> MSFTNVNYPASDGTVIFTEEQEALVVQSWNVMKKNSAELGLKLFLKIFEIAPTAKKMFSFVRDSDVPLEQNQKLKGHAMSVFVMTCKSAAQLRKAGKVTFGESSLKHMGSVHLKYGVVDEHFEVTRFALLETIKEAVPEMWSPEMKNAWAEAFNHLVAAIKAEMQR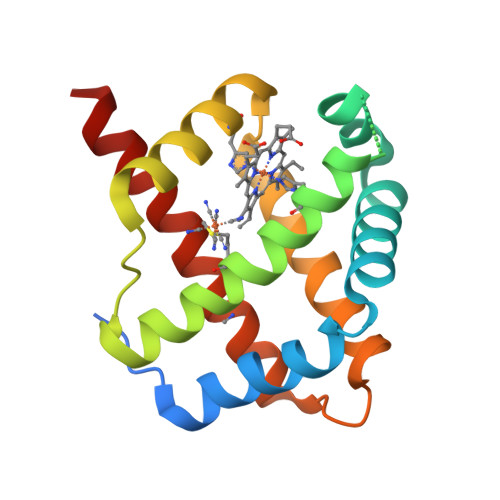LSTQP> MGNIGNLSAEKQISLYDGQPFISEQDVAAGDPNTPALTIEGPDGYVIAVDAGTPIAPEFRDSNGEKLDPSTRVIVQKCDRQGNPL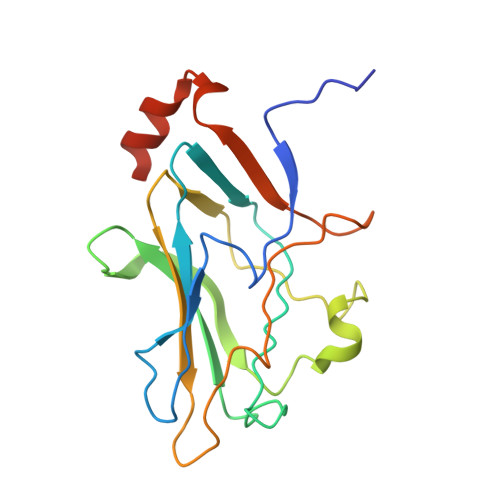GDGIIFNDTLGRFNYNKMRTDPDYMRKTAKSLMVDEREIVKVFVDVPDGANGYDAERSRFTLGDDTSDFGKAVEIVDHDDLTEGETQAVKSASQRSGGA Glyceraldehyde-3-phosphate dehydrogenase (GAPDH) is a highly conserved enzyme involved in the ubiquitous process of glycolysis and presents a loop (residues 208–215 of Escherichia coli GAPDH) in two alternative conformations (I and II). In the presence of inorganic phosphate (Pi), GAPDH catalyzes the conversion of D-glyceraldehyde-3-phosphate (G3P) to 1,3-diphosphoglycerate (BPG), accompanying the reduction of NAD+ to NADH. All the structures reported in this paper have four subunits: O, P, Q, and R. Each subunit contained two domains: the C-terminal catalytic domain and the N-terminal NAD+-binding domain. Two anion recognition sites, “Ps” and “Pi”, bind the C3 phosphate of G3P and inorganic phosphate, respectively.

The enzymatic activity of wild-type EcGAPDH1 was 3.84 × 104 times higher than that of C150S and 8.13 × 103 times higher than that of H177A. The analysis of the Q subunit of C150S.NAD.G3P and the O subunit of the thioacyl intermediate revealed that there are three differences. First, O1 of G3P is opposite to His177 in terms of its thioacyl intermediate structure, while it is oriented towards His177 in C150S.NAD.G3P. Second, the phosphate of G3P of the thioacyl intermediate is positioned in the “new Pi” site, while it is in the “Ps” site in C150S.NAD.G3P. Third, the loop that contains amino acid residues 208–215 is in conformation I in C150S.NAD.G3P, while it has two conformations in the thioacyl intermediate. In C150S.NAD.G3P, two hydrogen bonds are formed between O1 of G3P and Oγ of Thr209, while the O2 of G3P with the Nε of His177 strengthens the aldehyde form. However, these bonds do not exist in the hydrated form.

>[4x]HHHHHHSSGLVPRGSHMASMSKVGINGFGRIGRLVLRRLLEVKSNIDVVAINDLTSPKILAYLLKHDSNYGPFPWSVDFTEDSLIVDGKSIAVYAEKEAKNIPWKAKGAEIIVECTGFYTSAEKSQAHLDAGAKKVLISAPAGEMKTIVYNVNDDTLDGNDTIVSVASSTTNCLAPMAKALHDSFGIEVGTMTTIHAYTGTQSLVDGPRGKDLRASRAAAENIIPHTTGAAKAIGLVIPELSGKLKGHAQRVPVKTGSVTELVSILGKKVTAEEVNNALKQATTNNESFGYTDEEIVSSDIIGSHFGSVFDATQTEITAVGDLQLVKTVAWYDNEYGFVTQLIRTLEKFAKL> MRVFHFSKLPLGVAILAASSSVFAVTLDGGAVAAPDQYGAKVAAEILKKGGNAVDAAVATAFTLAVTYPEAGNIGGGGFMTLYVDGKPYFLDYREIAPKAATKTMYLNEKGEVIENLSLVGAKAAGVPGTVMGLWEAHQRFGKLKWSELLTPAIGYAQTGFKVADQQYQYRQDAIALFNGKTNFGDYFGTMKPGEVFKQPELAKTLERIADKGPDDFYKGETAKLLIAQMKQDGGLITSDDLVDYQAKWREPMRIDWQGNTLYTAPLPSSGGIALAQLIGIKEQRAADFKGVELNSAKYIHLLSEIEKRVFADRADYLGDPQFSKVPVAQLTDPKYIAKRAGEVNPDAISATEKVRPGLEPHQTTHFSIVD;> TTHFSIVDKDGNAVSNTYTLNWDFGSGVVVKGAGFLLNDEMDDFSSKPGVANAFGVVGSDANAIEPGKRMLSSMSPSIVTRDGHVSLVLGTPGGSRIFTSIFQVLNNVYDFHLPLEKAVAAQRVHHQLLPKDTIYYDAYAPLTGKVADELKAMGYTLEDQGWNMGDIQAIRVNGKALETASDP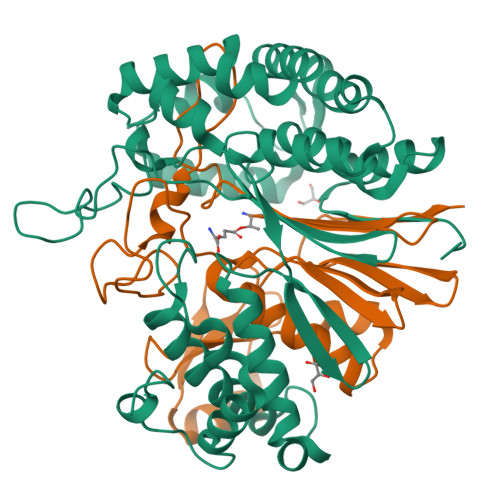RGRGVGMVVKP>AGKPVLHYFNARGRMECIRWLLAAAGVEFEEKFIQSPEDLEKLKKDGNLMFDQVPMVEIDGMKLVQTRAILNYIATKYDLYGKDMKERALIDMYTEGILDLTEMIGQLVLCPPDQREAKTALAKDRTKNRYLPAFEKVLKSHGQDYLVGNRLTRVDVHLLELLLY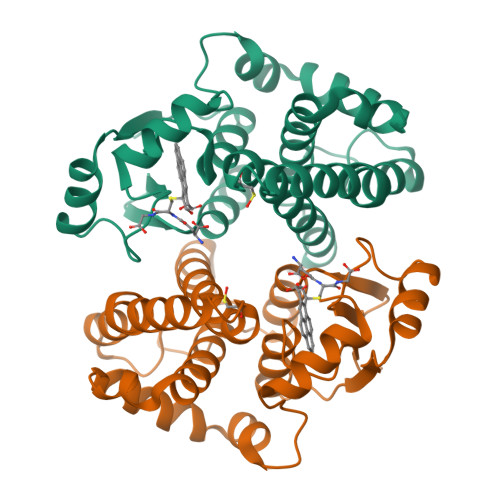VEELDASLLTPFPLLKAFKSRISSLPNVKKFLQPGSQRKPPLDAKQIEEARKVFKF[2x]Interestingly, DmCE1B in the D. mossii PUL 17 comprises two individual CE1 catalytic domains separated by a small CBM48 domain. To assess the role of each catalytic domain of the multicatalytic DmCE1B, the separate domains were also produced: DmCE1B_nt (45.3 kDa), comprising the N-terminal CE1 domain and the CBM48 domain, and DmCE1B_ct (43.3 kDa) comprising the CBM48 domain and the C-terminal CE1 domain. DmCE1B_ct forms two discrete globular domains, a ten-stranded β-sandwich domain consistent with the CBM48 family structure (residues 294–393) connected via a short linker (residues 394–404) to a three-layer αβα-sandwich (residues 405–656) typical of CE1 enzymes. Comparison to other CE1 family members enables annotation of the catalytic triad in DmCE1B_ct (Ser542, His638, Glu606), which is found in a groove between the CE1 and CBM48 domains.

Two protein molecules were present in the asymmetric unit and aligned along a noncrystallographic symmetry operator with the two α/β-hydrolase domains packed with β1 of their β-sheets adjacent and antiparallel to each other and the CBM48 domains clasping each other. The interaction in the dimer masks 10% of accessible surface, as determined by PISA, but with only a few key interactions suggesting the interaction might be biologically relevant. The two protomers showed high structural similarity to each other, with an all-atom root mean square deviation of 1.01 Å. Two stretches of residues in the α/β-hydrolase domain (residues 493–508 and 572–574) were unable to be modeled in both protomers likely owing to flexibility in these regions. A chloride ion was observed in the active site of the protein coordinating with the hydroxyl of the catalytic serine and the main chain amides of Gly450 and Met543, which likely comprise the oxyanion hole. No inhibition of DmCE1B_ct-mediated hydrolysis of 4-MU-Ac was observed in chloride concentrations up to 100 mM, indicating that the presence of the ion is likely an artifact of crystallization. In DmCE1B_ct, the positioning of the CBM48 domain relative to the CE1 domain is stabilized by hydrogen bonds through several residues: the main chain amide of Ser383 to the main chain carbonyl of Gly451, the hydroxyl of Tyr361 with an oxygen of the carboxylate of Glu452, the Nδ of His360 with both Oε1 and Oε2 of the carboxylate from Glu639, and a salt bridge between Glu390 and Arg644.

>[2x]MGSSHHHHHHSSENLYFQGHSEEAEVGISASTNIPGAQYPQILSGNRVLFRIKAPDAKRVQVDLGKKYDMVREEEGSWAITTDPIVEGFHYYSILIDGVAVCDPASRTFYGMSRMASGIEIPEEGVDYYNLKNVPHGQIRQIRYFSDVTKAWRRAFVYTPAGYDANTSQRYPVLYLQHGGGEDETGWPNQGKMDAIIDNLIAEGKAKPMIVVMDNGYAVDPSASSANSPQGLRGLFQNSALEKVFINEIIPLVDKEFRTIADRDHRAMAGLSMGGFQAFQIAMTNLDKFAYVGGFSGGGIIEQGGDFSKMYNNVWSDVDTFNKRVKLIYLSIGTAEPTNMYQTVNNFHKEFEKAGIKHVYYESPGTSHEWLTWRRSLNQFAELLFK> SKVVVPAQGKKITLQNGKLNVPENPIIPYIEGDGIGVDVTPAMLKVVDAAVEKAYKGERKISWMEIYTGEKSTQVYGQDVWLPAETLDLIREYRVAIKGPLTTPVGGGIRSLNVALRQELDLYICLRPVRYYQGTPSPVKHPEL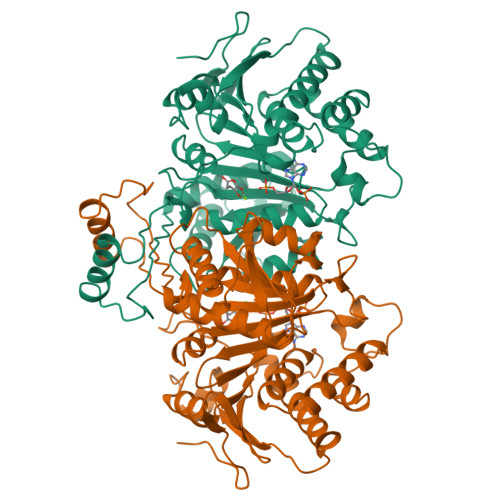TDMVIFRENSEDIYAGIEWKADSADAEKVIKFLREEMGVKKIRFPEHCGIGIKPCSEEGTKRLVRAAIEYAIANDRDSVTLVHKGNIMKFTEGAFKDWGYQLAREEFGGELIDGGPWLKVKNPNTGKEIVIKDVIADAFLQQILLRPAEYDVIACMNLNGDYISDALAAQVGGIGIAPGANIGDECALFEATHGTAPKYAGQDKVNPGSIILSAEMMLRHMGWTEAADLIVKGMEGAINAKTVTYDFERLMDGAKLLKCSEFGDAIIENM We have developed a functionalized, modular biomaterial formed by the controlled self-assembly of two proteins. The ZT polymer is composed of proteins of human origin produced recombinantly in bacteria. It is based on the naturally occurring complexation of the protein telethonin (Tel) with the two N-terminal immunoglobulin (Ig) domains, Z1Z2, from titin in the Z-disc of the muscle sarcomere. Specifically, its 90 N-terminal amino-acid residues become “sandwiched” between two antiparallel Z1Z2 doublets, forming a wing-like hairpin structure that builds an intermolecular β-sheet across the three components. The display of peptidic sequences on the ZT polymer is established, with sequences having been introduced both in Tel and Z1212 components without preventing polymerization. Both components permit fusing peptidic sequences to their N- and C-termini and, in addition, Z1212 permits the introduction of motifs in four internal positions, namely the CD loop of each of its four Ig domains.

However, they possess a surface exposed loop, the CD loop, which is a region of low sequence conservation. We have demonstrated that the CD loop can tolerate drastic diversification in length and composition and have established its suitability as a locus for peptide grafting. In the Z1Z2 variant carrying the decorin motif KLER in the CD loop of Z1 (Z12KLER), the motif replaced five native residues so as to become inserted between residues V45 and L51. This insertion point was chosen as the V and L residues in Z1 corresponded to the natural flanking residues of KLER in decorin (VKLERL). Decorin is a protein associated with cartilage homeostasis that binds to collagens and plays a role in their stability, organization, and fibrillogenesis. In decorin, the KLER motif is located within a loop of the leucine-rich repeat 3, the region that binds collagen and the incorporation of this sequence in a PEG-peptide co-polymer promoted chondrogenesis of human mesenchymal stromal cells. It was envisioned that the CD loop would constitute a structurally suitable area to incorporate the KLER sequence. Interestingly, the overall pattern of exposed Lys, Glu, and Arg side chains with a buried Leu sidechain is preserved in Z12KLER, but the main chain adopts a slight helical turn that causes the side chains to be positioned closer together producing a compacter KLER motif than that of decorin. Given that loop sequences can undergo changes induced by their binding targets, it remains to be established whether the observed difference affects the biological function of the engineered motif. In conclusion, data on the various variants establish the suitability of the CD loop as a locus for peptide grafting, capable of supporting the display of bioactive peptidic motifs on the ZT polymer.

>GAMATQAPTFTQPLQSVVVLEGSTATFEAHISGFPVPEVSWFRDGQVKLERLPGVQISFSDGRAKLTIPAVTKANSGRYSLKATNGSGQATSTAELLVKAETAPPNFVQRLQSMTVRQGSQVRLQVRVTGIPTPVVKFYRDGAEIQSSLDFQISQEGDLYSLLIAEAYPEDSGTYSVNATNSVGRATSTAELLVQGE[5x]>[9x]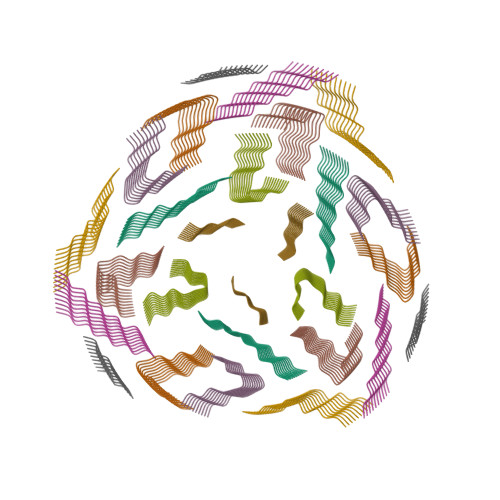DLIIKGISVHI>AKLLIPQAASAIEQMKLEIASEFGVQLGAETTSRANGSVGGEITKRLVRLA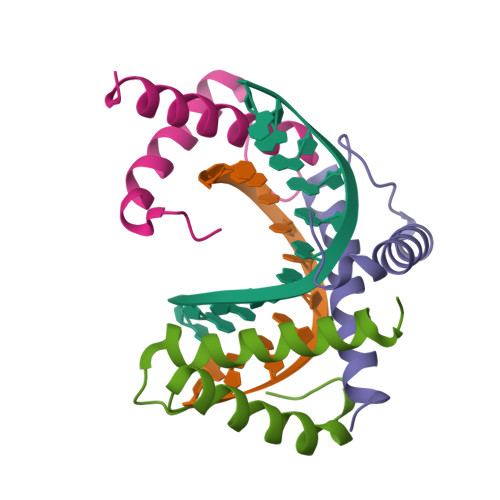QQNMGGQFHGQQ[3x]> NWVDITQDFEEACRELKLGELLHDKLFGLFEAMSAIEMMDPKMDAGMIGNQVNRKVLNFEQAIKDGTIKIKDLTLPELIGIMDTCFCCLITWLEGHSLAQTVFTCLYIHNPDFIEDPAMKAFALGILKICDIAREKVNKAAVFEEEDFQSMTYGFKMANSVTDLRVTGMLKDVEDDMQRRVKS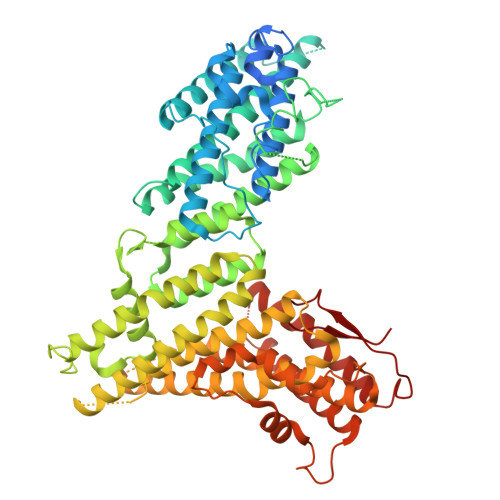TRSRQGEERDPEVELEHQQCLAVFSRVKFTRVLLTVLIAFTKKETSAVAEAQKLMVQAADLLSAIHNSLHHGIQAQNDTTKGDHPIMMGFEPLVNQRLLPPTFPRYAKIIKREEMVNYFARLIDRIKTVCEVVNLTNLHCILDFFCEFSEQSPCVLSRSLLQTTFLVDNKKVFGTHLMQDMVKDALRSFVSPPVLSPKCYLYNNHQAKDCIDSFVTHCVRPFCSLIQIHGHNRARQRDKLGHILEEFATLQDEAEKVDAALHTMLLKQEPQRQHLACLGTWVLYHNLRIMIQYLLSGFELELYSMHEYYYIYWYLSEFLYAWLMSTLSRADGSQMAEERIMEEQQKGRSSKKTKKKKKVRPLSREITMSQAYQNMCAGMFKTMVAFDMDGKVRKPKFELDSEQVRYEHRFAPFNSVMTPPPVHYLQFKEMSDLNKYSPPPQSPELYVAASKHFQQAKMILENIPNPDHEVNRILKVAKPNFVVMKLLAGGHKKESKVPPEFDFSAHKYFPVVKLV>MEGFPVRVRVDVRFRD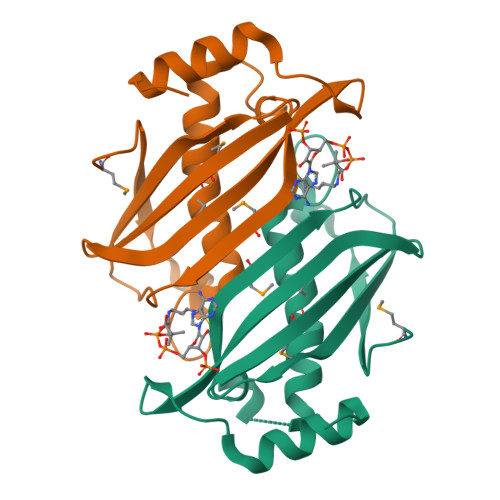LDPLGHVNNAVFLSYMELARIRYFQRISPDWLEEGHFVVARMEVDYLRPILLGDEVFVGVRTVGLGRSSLRMEHLVTANGESAAKGLGVLVWLEGGRPAPLPEAIRERIRALEGRPL[4x]>GSMASSDTEGKRVVVIGGGLVGALNACFLAKRNFQVDVYEAREDIRVANFMRGRSINLALSYRGRQALKAVGLEDQIVSKGVPMKARMIHSLSGKKSAIPYGNKSQYILSISREKLNKDLLTAVESYPNAKVHFGHKLSKCCPEEGILTMLGPNKVPRDITCDLIVGCDGAYSTVRAHLMKKPRFDYSQQYIPHGYMELTIPPKNGEYAMEPNCLHIWPRNAFMMIALPNMDKSFTCTLFMSFEEFEKLPTHSDVLDFFQKNFPDAIPLMGEQALMRDFFLLPAQPMISVKCSPFHLKSRCVLMGDAAHAIVPFFGQGMNAGFEDCLVFDELMDKFNNDLSVCLPEFSRFRIPDDHAISDLSMYNYIEMRAHVNSRWFLFQRLLDKFLHALMPSTFIPLYTMVAFTRIRYHEAVLRWHWQKKVINRGLFVLGSLVAIGSAYILVHHLSPRPLELLRSAWTGTSGHWNRSADISPRVPWSHENLYFQGDYKDDDDK[2x]

KMO is a class A flavoprotein monooxygenase, which catalyses the hydroxylation of L-kynurenine to 3-hydroxykynurenine (3-HK). We determined the full-length structure of Rat-KMO in its membrane-embedded form complexed with compound 3 and compound 4 at 3.0 Å resolution. Unexpectedly, the crystal structure showed that the C-terminal region was comprising only one transmembrane domain, with the other predicted transmembrane helix lying laterally along the membrane. The KMO monomers are linked by intermolecular β-sheets at F183-Y189 (β12), strongly suggesting physiological dimerisation.

Furthermore, introduction of a benzyloxy group at the 2-position of benzoic acid led to a dramatic increase in KMO potency, especially in the rat homolog (compound 3). Optimisation of 1 produced a potent inhibitory compound, 3, for which the crystal structure was determined. The ligand-binding pocket of the full-length Rat-KMO was composed not only of residues from the FAD-binding domain but also of residues from the C-terminal region. Surprisingly, R380, a residue from this C-terminal region, formed hydrogen bonds with the carboxylic acid moiety of compound 3. Compound 3 was recognised by hydrogen bonds on one side by residues R85, Y99, R380 and Y398. On the other side, the chlorofluorophenyl group and benzyloxy group formed hydrophobic interactions with surrounding residues I215, M222, I224, F312, V371, M367, and F376. The hydrophobic interactions may explain the remarkably low koff values in surface plasmon resonance experiments. No strong contacts between FAD and compound 3 were observed. Five residues in the C-terminal region starting from K380 differed from that in Rat-KMO. This sequence discrepancy likely underlies the difference in potency between these species, as shown in Table 1.> AKNIKKGPAPFYPLEDGTAGEQLHKAMKRYALVPGTIAFTDAHIEVNITYAEYFEMSVRLAEAMKRYGL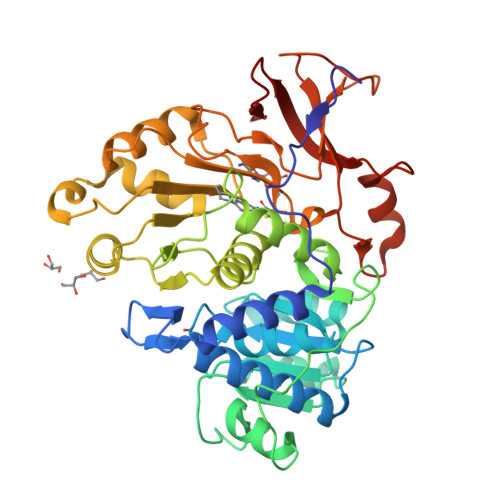NTNHRIVVCSENSLQFFMPVLGALFIGVAVAPANDIYNERELLNSMNISQPTVVFVSKKGLQKILNVQKKLPIIQKIIIMDSKTDYQGFQSMYTFVTSHLPPGFNEYDFVPESFDRDKTIALIMNSSGSTGLPKGVALPHRTACVRFSHARDPIFGNQIIPDTAILSVVPFHHGFGMFTTLGYLICGFRVVLMYRFEEELFLRSLQDYKIQSALLVPTLFSFFAKSTLIDKYDLSNLHEIASGGAPLSKEVGEAVAKRFHLPGIRQGYGLTETTSAILITPEGDDKPGAVGKVVPFFEAKVVDLDTGKTLGVNQRGELCVRGPMIMSGYVNNPEATNALIDKDGWLHSGDIAYWDEDEHFFIVDRL> SQIRQNYSTEVEAAVNRLVNL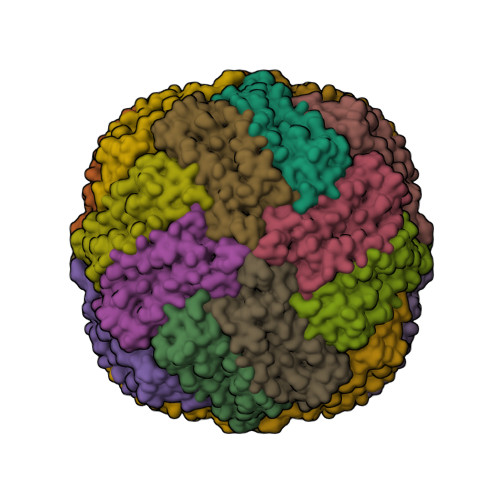YLRASYTYLSLGFYFDRDDVALEGVCHFFRELAEEKREGAERLLKMQNQRGGRALFQDLQKPSQDEWGTTLDAMKAAIVLEKSLNQALLDLHALGSAQADPHLCDFLESHFLDEEVKLIKKMGDHLTNIQRLVGSQAGLGEYLFERLTLK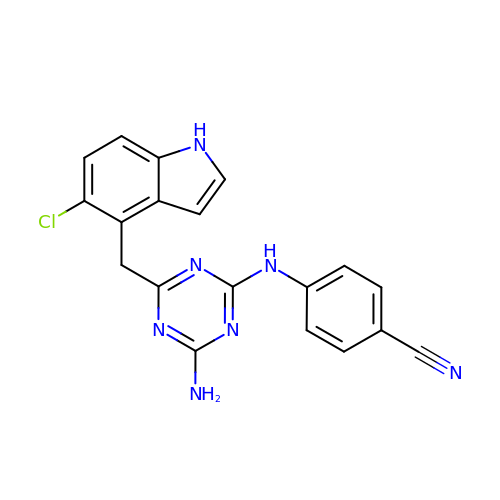4-[4-AMINO-6-(5-CHLORO-1H-INDOL-4-YLMETHYL)-[1,3,5]TRIAZIN-2-YLAMINO]-BENZONITRILE | C19 H14 Cl N7 | SOKOHDQTKSROQZ-UHFFFAOYSA-N>GSFKFTAQQHVYDINGVKVGGQPGEYPTVLIGSIFYR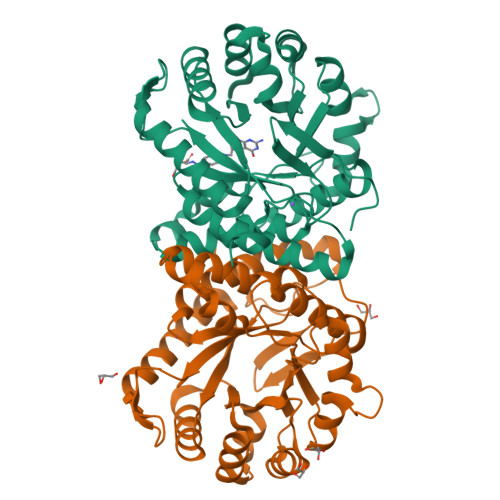GHKIVSDGQKGIFDKDAAKALLDQEAELSAETGNPFIIDVLGESVEALTKYVEFILENTTAPFLLDSISPDVRVGALKNLGKDPEIQKRLIYNSIEEHYTEEELAAIKEAGLKTAVILAFSKKALKPNARIDLLQGKDDKEGLIAAAKRAGIEQFLVDPGVLDVASNSWTTEAINVVKEQFGYPGGCAPSNAVYLWKKMRSKGTPFFEVAGAAVFTYPITQGADFILYGPMMNAPWVYRAIATTDAMIAYNNKLTGVKMGTTEHPLLKIF[2x]> SMPFPEGKVLDDMEGNQWVLGKKIGSGGFGLIYLAFPTNKPEKDARHVVKVEYQENGPLFSELKFYQRVAKKDCIKKWIERKQLDYLGIPLFYGSGLTEFKGRSYRFMVMERLGIDLQKISGQNGTFKKSTVLQLGIRMLDVLEYIHENEYVHGDIKAANLLLGYKNPDQVYLADYGLSYRYCPNGNHKQYQENPRKGHNGTIEFTSLDAHKGVALSR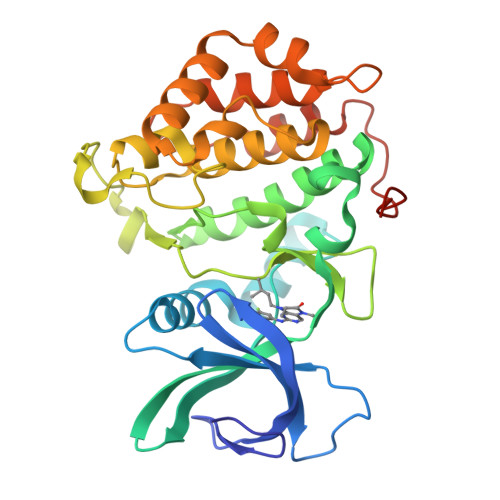RSDVEILGYCMLRWLCGKLPWEQNLKDPVAVQTAKTNLLDELPQSVLKWAPSGSSCCEIAQFLVCAHSLAYDEKPNYQALKKILNPHGIPLGPLDFSTKGQSINVH6-CHLOROPURINE 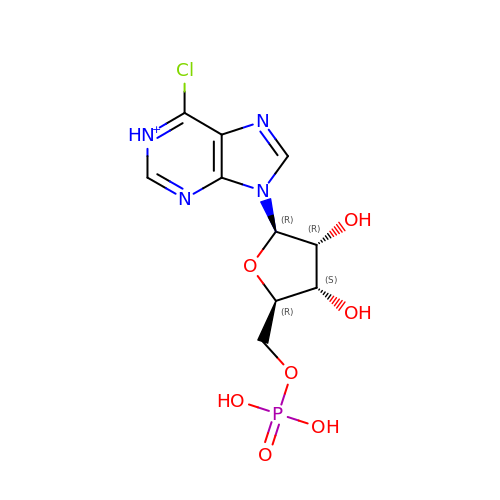RIBOSIDE, 5'-MONOPHOSPHATE | C10 H13 Cl N4 O7 P | ALOBOMYIOYNCBS-KQYNXXCUSA-O> MSLTEQIEQFASRFRDDDATLQSRYSTLSELYDIMELLNSPEDYHFFLQAVIPLLLNQLKEVPISYDAHSPEQKLRNSMLDIFNRCLMNQTFQPYAMEVLEFLLSVLPKENEENGILCMKVLTTLFKSFKSILQDKLDSFIRIIIQIYKNTPNLINQTFYEAGKAEQGDLDSPKEPQADELLDEFSKNDEEKDFPSKQSSTEPRFENSTSSNGLRSSMFSFKILSECPITMVTLYSSYKQLTSTSLPEFTPLIMNLLNIQIKQQQEAREQAESRGEHFTSISTEIINRPAYCDFILAQIKATSFLAYVFIRGYAPEFLQDYVNFVPDLIIRLLQDCPSELSSARKELLHATRHILSTNYKKLFLPKLDYLFDERILIGNGFTMHETLRPLAYSTVADFIHNIRSELQLSEIEKTIKIYTGYLLDESLALTVQIMSAKLLLNLVERILKLGKENPQEAPRAKKLLMIIIDSYMNRFKTLNRQYDTIMKYYGRYETHKKEKAEKLKNSIQDNDKESEEFMRKVLEPSDDDHLMPQPKKEDINDSPDVEMTESDKVVKNDVEMFDIKNYAPILLLPTPTNDPIKDAFYLYRTLMSFLKTIIHDLKVFNPPPNEYTVANPKLWASVSRVFSYEEVIVFKDLFHECIIGLKFFKDHNEKLSPETTKKHFDISMPSLPVSATKDARELMDYLAFMFMQMDNATFNEIIEQELPFVYERMLEDSGLLHVAQSFLTSEITSPNFAGILLRFLKGKLKDLGNVDFNTSNVLIRLFKLSFMSVNLFPNINEVVLLPHLNDLILNSLKYSTTAEEPLVYFYLIRTLFRSIGGGRFENLYRSIKPILQVLLQSLNQMILTARLPHERELYVELCITVPVRLSVLAPYLPFLMKPLVFALQQYPDLVSQGLRTLELCIDNLTAEYFDPIIEPVIDDVSKALFNLLQPQPFNHAISHNVVRILGKLGGRNRQFLKPPTDLTEKTELDIDAIADFKINGMPEDVPLSVTPGIQSALNILQSYKSDIHYRKSAYKYLTCVLLLMTKSSAEFPTNYTELLKTAVNSIKLERIGIEKNFDLEPTVNKRDYSNQENLFLRLLESVFYATSIKELKDDAMDLLNNLLDHFCLLQVNTTLLNKRNYNGTFNIDLKNPNFMLDSSLILDAIPFALSYYIPEVREVGVLAYKRIYEKSCLIYGEELALSHSFIPELAKQFIHLCYDETYYNKRGGVLGIKVLIDNVKSSSVFLKKYQYNLANGLLFVLKDTQSEAPSAITDSAEKLLIDLLSITFADVKEEDLGNKVLENTLTDIVCELSNANPKVRNACQKSLHTISNLTGIPIVKLMDHSKQFLLSPIFAKPLRALPFTMQIGNVDAITFCLSLPNTFLTFNEELFRLLQESIVLADAEDESLSTNIQKTTEYSTSEQLVQLRIACIKLLAIALKNEEFATAQQGNIRIRILAVFFKTMLKTSPEIINTTYEALKGSLAENSKLPKELLQNGLKPLLMNLSDHQKLTVPGLDALSKLLELLIAYFKVEIGRKLLDHLTAWCRVEVLDTLFGQDLAEQMPTKIIVSIINIFHLLPPQADMFLNDLLLKVMLLERKLRLQLDSPFRTPLARYLNRFHNPVTEYFKKNMTLRQLVLFMCNIVQRPEA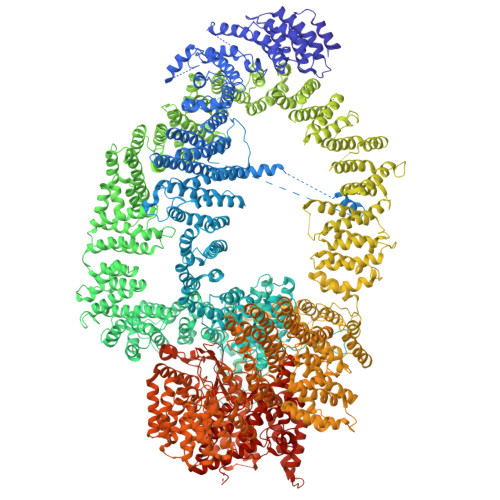KELAEDFEKELDNFYDFYISNIPKNQVRVVSFFTNMVDLFNTMVITNGDEWLKKKGNMILKLKDMLNLTLKTIKENSFYIDHLQLNQSIAKFQALYLRFTELSERDQNPLLLDFIDFSFSNGIKASYSLKKFIFHNIIASSNKEKQNNFINDATLFVLSDKCLDARIFVLKNVINSTLIYEVATSGSLKSYLVEDKKPKWLELLHNKIWKNSNAILAYDVLDHHDLFRFELLQLSAIFIKADPEIIAEIKKDIIKFCWNFIKLEDTLIKQSAYLVTSYFISKFDFPIKVVTQVFVALLRSSHVEARYLVKQSLDVLTPVLHERMNAAGTPDTWINWVKRVMVENSSSQNNILYQFLISHPDLFFNSRDLFISNIIHHMNKITFMSNSNSDSHTLAIDLASLILYWENKTLEITNVNNTKTDSDGDVVMSDSKSDINPVEADTTAIIVDANNNSPISLHLREACTAFLIRYVCASNHRAIETELGLRAINILSELISDKHWTNVNVKLVYFEKFLIFQDLDSENILYYCMNALDVLYVFFKNKTKEWIMENLPTIQNLLEKCIKSDHHDVQEALQKVLQVIMKAIKAQGVSVIIEEESPGKTFIQMLTSVITQDLQETSSVTAGVTLAWVLFMNFPDNIVPLLTPLMKTFSKLCKDHLSISQPKDAMALEEARITTKLLEKVLYILSLKVSLLGDSRRPFLSTVALLIDHSMDQNFLRKIVNMSRSWIFNTEIFPTVKEKAAILTKMLAFEIRGEPSLSKLFYEIVLKLFDQEHFNNTEITVRMEQPFLVGTRVEDIGIRKRFMTILDNSLERDIKERLYYVIRDQNWEFIADYPWLNQALQLLYGSFNREKELSLKNIYCLSPPSILQEYLPENAEMVTEVNDLELSNFVKGHIASMQGLCRIISSDFIDSLIEIFYQDPKAIHRAWVTLFPQVYKSIPKNEKYGFVRSIITLLSKPYHTRQISSRTNVINMLLDSISKIESLELPPHLVKYLAISYNAWYQSINILESIQSNTSIDNTKIIEANEDALLELYVNLQEEDMFYGLWRRRAKYTETNIGLSYEQIGLWDKAQQLYEVAQVKARSGALPYSQSEYALWEDNWIQCAEKLQHWDVLTELAKHEGFTDLLLECGWRVADWNSDRDALEQSVKSVMDVPTPRRQMFKTFLALQNFAESRKGDQEVRKLCDEGIQLSLIKWVSLPIRYTPAHKWLLHGFQQYMEFLEATQIYANLHTTTVQNLDSKAQEIKRILQAWRDRLPNTWDDVNMWNDLVTWRQHAFQVINNAYLPLIPALQQSNSNSNINTHAYRGYHEIAWVINRFAHVARKHNMPDVCISQLARIYTLPNIEIQEAFLKLREQAKCHYQNMNELTTGLDVISNTNLVYFGTVQKAEFFTLKGMFLSKLRAYEEANQAFATAVQIDLNLAKAWAQWGFFNDRRLSEEPNNISFASNAISCYLQAAGLYKNSKIRELLCRILWLISIDDASGMLTNAFDSFRGEIPVWYWITFIPQLLTSLSHKEANMVRHILIRIAKSYPQALHFQLRTTKEDFAVIQRQTMAVMGDKPDTNDRNGRRQPWEYLQELNNILKTAYPLLALSLESLVAQINDRFKSTTDEDLFRLINVLLIDGTLNYNRLPFPRKNPKLPENTEKNLVKFSTTLLAPYIRPKFNADFIDNKPDYETYIKRLRYWRRRLENKLDRASKKENLEVLCPHLSNFHHQKFEDIEIPGQYLLNKDNNVHFIKIARFLPTVDFVRGTHSSYRRLMIRGHDGSVHSFAVQYPAVRHSRREERMFQLYRLFNKSLSKNVETRRRSIQFNLPIAIPLSPQVRIMNDSVSFTTLHEIHNEFCKKKGFDPDDIQDFMADKLNAAHDDALPAPDMTILKVEIFNSIQTMFVPSNVLKDHFTSLFTQFEDFWLFRKQFASQYSSFVFMSYMMMINNRTPHKIHVDKTSGNVFTLEMLPSRFPYERVKPLLKNHDLSLPPDSPIFHNNEPVPFRLTPNIQSLIGDSALEGIFAVNLFTISRALIEPDNELNTYLALFIRDEIISWFSNLHRPIIENPQLREMVQTNVDLIIRKVAQLGHLNSTPTVTTQFILDCIGSAVSPRNLARTDVNFMPWF> MILDTDYITEDGKPVIRIFKKENGEFKIDYDRNFEPYIYALLKDDSAIEDVKKITAERHGTTVRVVRAEKVKKKFLGRPIEVWKLYFTHPQDQPAIRDKIKEHPAVVDIYEYDIPFAKRYLIDKGLIPMEGDEELKMLAFAIATLYHEGEEFAEGPILMISYADEEGARVITWKNIDLPYVDVVSTEKEMIKRFLKVVKEKDPDVLITYNGDNFDFAYLKKRSEKLGVKFILGREGSEPKIQRMGDRFAVEVKGRIHFDLYPVIRRTINLPTYTLEAVYEAIFGQPKEKVYAEEIAQAWETGEGLERVARYSMEDAKVTYELGKEFFPMEAQLSRLVGQSLWDVSRSSTGNLVEWFLLRKAYERNELAPNKPDERELARRRESYAGGYVKEPERGLWENIVYLDFRSLYPSIIITHNVSPDTLNREGCEEYDVAPQVGHKFCKDFPGFIPSLLGDLLEERQKVKKKMKATIDPIEKKLLDYRQRLIKILANSFYGYYGYAKARWYCKECAESVTAWGRQY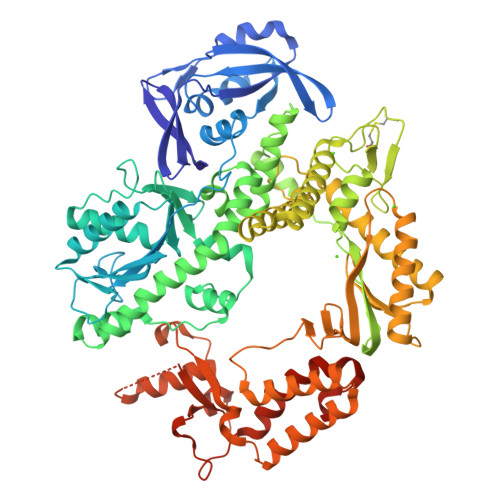IETTIREIEEKFGFKVLYADTDGFFATIPGADAETVKKKAKEFLDYINAKLPGLLELEYEGFYKRGFFATKKKYAVIDEEDKITTRGLKMVRRDWSEIAKETQARVLEAILKHGDVEEAVRIVKEVTEKLSKYEVPPEQLVIYQPITKQLHDYRARGPHVSVAKRLAARGIKIRPGTVISYIVPKGSGRIGDRAIPFDEFDPAKHKYDAGYYIENQVLPAVERILRAFGYRKEDLRYQKTRQVGLGAWLKPKT> MAFWTQLMLLLWKNFMYRRRQPVQLLVELLWPLFLFFILVAVRHSHPPLEHHECHFPNKPLPSAGTVPWLQGLICNVNNTCFPQLTPGEEPGRLSNFNDSLVSRLLADARTVLGGASAHRTLAGLGKLIATLRAARSTAQPQPTKQSPLEPPMLDVAELLTSLLRTESLGLALGQAQEPLHSLLEAAEDLAQELLALRSLVELRALLQRPRGTSGPLELLSEALCSVRGPSSTVGPSLNWYEASDLMELVGQEPESALPDSSLSPACSELIGALDSHPLSRLLWRRLKPLILGKLLFAPDTPFTRKLMAQVNRTFEELTLLRDVREVWEMLGPRIFTFMNDSSNVAMLQRLLQMQDEGRRQPRPGGRDHMEALRSFLDPGSGGYSWQDAHADVGHLVGTLGRVTECLSLDKLEAAPSEAALVSRALQLLAEHRFWAGVVFLGPEDSSDPTEHPTPDLGPGHVRIKIRMDIDVVTRTNKIRDRFWDPGPAADPLTDLRYVWGGFVYLQDLVERAAVRVLSGANPRAGLYLQQMPYPCYVDDVFLRVLSRSLPLFLTLAWIYSVTLTVKAVVREKETRLRDTMRAMGLSRAVLWLGWFLSCLGPFLLSAALLVLVLKLGDILPYSHPGVVFLFLAAFAVATVTQSFLLSAFFSRANLAAACGGLAYFSLYLPYVLCVAWRDRLPAGGRVAASLLSPVAFGFGCESLALLEEQGEGAQWHNVGTRPTADVFSLAQVSGLLLLDAALYGLATWYLEAVCPGQYGIPEPWNFPFRRSYWCGPRPPKSPAPCPTPLDPKVLVEEAPPGLSPGVSVRSLEKRFPGSPQPALRGLSLDFYQGHITAFLGHNGAGKTTTLSILSGLFPPSGGSAFILGHDVRSSMAAIRPHLGVCPQYNVLFDMLTVDEHVWFYGRLKGLSAAVVGPEQDRLLQDVGLVSKQSVQTRHLSGGMQRKLSVAIAFVGGSQVVILDEPTAGVDPASRRGIWELLLKYREGRTLILSTHHLDEAELLGDRVAVVAGGRLCCCGSPLFLRRHLGSGYYLTLVKARLPLTTNEKADTDMEGSVDTRQEKKNGSQGSRVGTPQLLALVQHWVPGARLVEELPHELVLVLPYTGAHDGSFATLFRELDTRLAELRLTGYGISDTSLEEIFLKVVEECAADTDMEDGSCGQHLCTGIAGLDVTLRLKMPPQETALENGEPAGSAPETDQGSGPDAVGRVQGWALTRQQLQALLLKRFLLARRSRRGLFAQIVLPALFVGLALVFSLIVPPFGHYPALRLSPTMYGAQVSFFSEDAPGDPGRARLLEALLQEAGLEEPPVQHSSHRFSAPEVPAEVAKVLASGNWTPESPSPACQCSRPGARRLLPDCPAAAGGPPPPQAVTGSGEVVQNLTGRNLSDFLVKTYPRLVRQGLKTKKWVNEVRYGGFSLGGRDPGLPSGQELGRSVEELWALLSPLPGGALDRVLKNLTAWAHSLDAQDSLKIWFNNKGWHSMVAFVNRASNAILRAHLPPGPARHAHSITTLNHPLNLTKEQLSEGALMASSVDVLVSICVVFAMSFVPASFTLVLIEERVTRAKHLQLMGGLSPTLYWLGNFLWDMCNYLVPACIVVLIFLAFQQRAYVAPANLPALLLLLLLYGWSITPLMYPASFFFSVPSTAYVVLTCINLFIGINGSMATFVLELFSDQKLQEVSRILKQVFLIFPHFCLGRGLIDMVRNQAMADAFERLGDRQFQSPLRWEVVGKNLLAMVIQGPLFLLFTLLLQHRSQLLPQPRVRSLPLLGEEDEDVARERERVVQGATQGDVLVLRNLTKVYRGQRMPAVDRLCLGIPPGECFGLLGVNGAGKTSTFRMVTGDTLASRGEAVLAGHSVAREPSAAHLSMGYCPQSDAIFELLTGREHLELLARLRGVPEAQVAQTAGSGLARLGLSWYADRPAGTYSGGNKRKLATALALVGDPAVVFLDEPTTGMDPSARRFLWNSLLAVVREGRSVMLTSHSMEECEALCSRLAIMVNGRFRCLGSPQHLKGRFAAGHTLT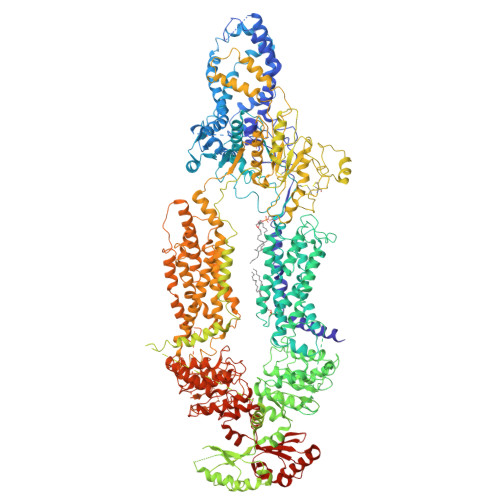LRVPAARSQPAAAFVAAEFPGAELREAHGGRLRFQLPPGGRCALARVFGELAVHGAEHGVEDFSVSQTMLEEVFLYFSKDQGKDEDTEEQKEAGVGVDPAPGLQHPKRVSQFLDDPSTAETVL> MSSDVKDSSHLEKQNSQEYSNSKQNGEIDIMEMLPQKKMYIIEKQFDQSGKGLKIDEFVRVMLTHLDFDKSDVQKEDQITLALIDLFKEIDVNGDGTMEWEEFSDHIISLGLLRNDRSFKNVIKNYFPSEHIKDNQKHETPIEKIVYFDKLKYLVVLEKDSTRFKVYNANTAELYYEVNAHKCAVLDAEYIPDQNLIATSSNDLTINFWDSSFFIPKQIVSVPEIQLCMRYAKWSTQSQPTYLYTGGSDSIIHIYDTKTLKEKGTIGGWNPFFKRDSQQYGHASPIGDILPINIQTTLVTAGLDANICLWDAATHLPKKELRGHEKGVYSLDWSDFSPMNQCLLSAGLDHEAFVWNTYVKEKIFLLRGHNHPLIGVKCLPGTPQVITADINGMVKVWDVRNFLCMQTINVPTDELNSFVVTSNQKKRIIFGARRLYYYEYDEPKDQMLTDEKMCLRVLYNSVLLCLITLHPDCIKVWDIRTGKLQSVYRELSTAELTVCVLDTRKRKLFVGDADGNIFTVNIKNGAKMKKFEKHNNRMITDLTHWTSKKPATIEIGGDDDDEDGTGDSRRVVSCSREETVFIHDEDSSDPSRSCRYKMKQHKSSVNSLSLKQDSELFASASDDGNIVITNLNSYRQETLPSTQYPFEKKKVIFLDPYNALVTSDSEGYVHFYCVNNGKARTRYLLTKKYETTSVVNNKVDKFPVTHLAFNSDNNMLLLSDELGNVTIWDLTIFLKKLDEIKDDNIQQQKTKQAQTPLKQTPNRASNGFFPTELDELKQINEKQISLSQMDNLEKYFQDKDIAFVHQLKGAHNDGITWIEVLKEYNMFATSSFDCCCHLWSF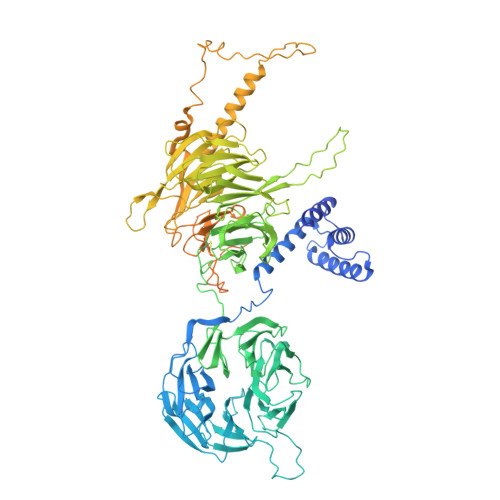NDYKKMGSLILGHDIMNNNWQLRVDEEKRKVDAQYYMEKLKKKLNKDDQSDDEEKNSQKQDESMMSDKNFDQKNQKKPKKTEKGEKGEKAPEKPLPEKKKVLTAQEKMEQNKKLKNELKLEFDPALLNLNKNKKQVLSEKEQIEKASELLEKVKKFNDVIANKNKDRRNPLEIDYDDFLRAYQMDEQVDIYLDQNEEEEEDNNILYDLDDPKNQSIPAGAYTSKGAFKSKNIGRKNKI> GSDELYRQSLEIISRYLREQATGAKDTKPMGRSGATSRKALETLRRVGDGVQRNHETAFQGMLRK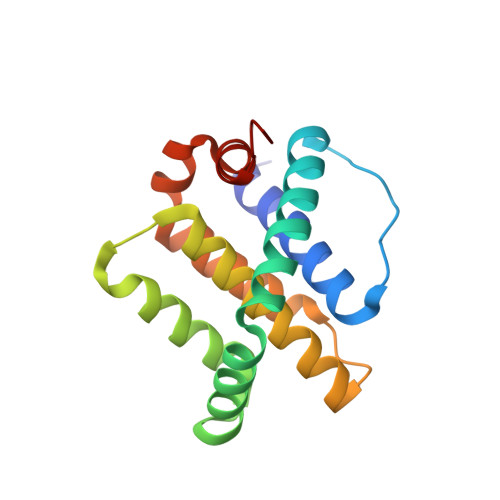LDIKNEDDVKSLSRVMIHVFSDGVTNWGRIVTLISFGAFVAKHLKTINQESCIEPLAESITDVLVRTKRDWLVKQRGWDGFVEFFHVEDLE>[4x]MNDSSVIYRAIVTSKFRTEKMLNFYNSIGSGPDKNTIFITFGRSEPWSSNENEVGFAPPYPTDSVLGVTDMWTHMMGTVKVLPSMLDAVIPRRDWGDTRYPDPYTFRINDIVVCNSAPYNATESGAGWLVYRCLDVPDTGMCSIASLTDKDECLKLGGKWTPSARSMTPPEGRGDAE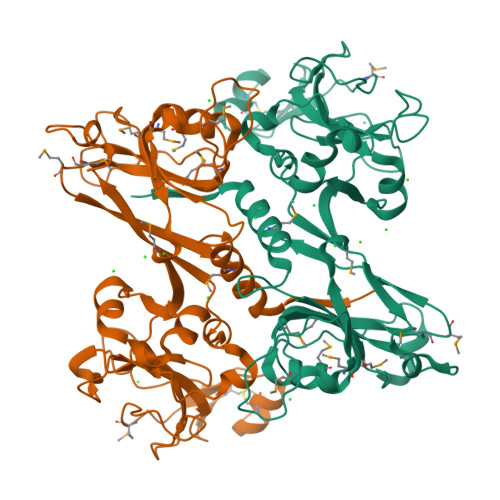GTIEPGDGYVWEYLFEIPPDVSINRCTNEYIVVPWPEELKEDPTRWGYEDNLTWQQDDFGLIYRVKANTIRFKAYLDSVYFPEAALPGNKGFRQISIITNPLEAKAHPNDPNVKAEKDYYDPEDLMRHSGEMIYMENRPPIIMAMDQTEEINILFTF>[2x]MKCTKNALAQTGFNKDKYFNGDVWYV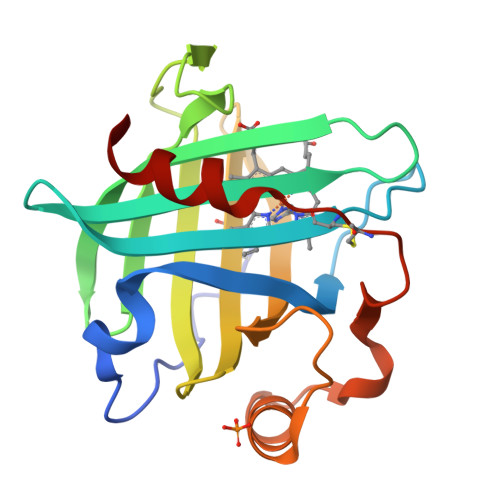TDYLDLEPDDVPKRYCAALAAGTASGKLKEALYCYDPKTQDTFYDVSELQEESPGKYTANFKKVEKNGNVKVDVTSGNYYTFTVMYADDSSALIHTCLHKGNKDLGDLYAVLNRNKDTNAGDKVKGAVTAASLKFSDFISTKDNKCEYDNVSLKSLLTK> MSVVTKSIVNADAEARYLSPGELDR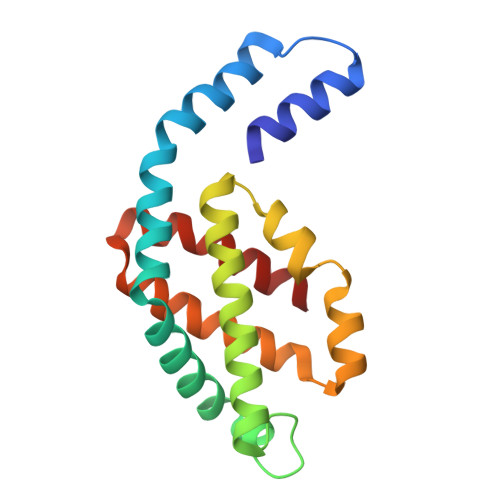IKNFVSTGERRLRIAQTLTENRERIVKQAGDQLFQKRPDVVSPGGNAYGEEMTATCLRDLDYYLRLVTYGIVAGDVTPIEEIGLVGVREMYNSLGTPIPAVAEGIRAMKNVACSLLSAEDAAEAGSYFDFVIGAMQ>ATKEGRVQKYAKERFEALGGLVRKLSYEGRSGAPDLLVILPRGVIWFVEVKKDENTKPDPHQLREHERFRKRGANVFVVGSFKQVDKLIEHYY[2x]

However, we were able to solve the first VRR-Nuc domain structures using single-domain proteins derived from three bacteria and bacteriophage as surrogates: Psychrobacter (psNUC); Streptococcus equi bacteriophage P9 (stNUC); and Salmonella enteritidis typing phage 3 (saNUC). Crystal structures of three representatives show that they structurally resemble Holliday junction resolvases (HJRs), are dimeric in solution, and are able to cleave symmetric four-way junctions. DALI searches show that the structures with greatest similarity to the VRR-Nuc domains are all Holliday-junction-resolving enzymes exemplified by Hjc. As dimers, bacterial VRR-Nuc domains have two active sites and a DNA-binding surface with 2-fold symmetry that are well suited to the recognition and symmetrical, bilateral cleavage of Holliday junctions.

saNUC was solved by molecular replacement using the stNUC structure as a search model, revealing a dimeric arrangement of two molecules in the AU essentially identical to that seen in the stNUC crystals. Despite only having 34% sequence identity with stNUC, both have core structures that are remarkably similar (root-mean-square deviation = 1.3 Å over 86 Cα) and the orientation of active site residues is essentially identical to stNUC. By contrast to the other proteins, saNUC only formed nonspecific, higher-order complexes. stNUC and saNUC exhibited weaker nuclease activity against the Jbm5 HJ substrate, detectable only at protein concentrations above 1 μM and with increased reaction times. Under these conditions, stNUC showed robust activity, whereas cleavage by saNUC was much reduced. This suggests that our saNUC preparations have a low active fraction potentially also explaining the lack of structure selectivity seen in the gel mobility shift experiments. Whether the levels of activity observed for stNUC and saNUC are representative of those in vivo is unclear, but it would appear unlikely given their close structural homology to psNUC. Crucially, however, both enzymes retain the ability to produce symmetric cleavages within a HJ substrate, an activity that is not characteristic of VRR-Nuc domains within the FAN1 orthologs.4-azanyl-6-[1-(2-morpholin-4-ylethyl)pyrazol-4-yl]pyrimidine-5-carbonitrile | C14 H17 N7 O | 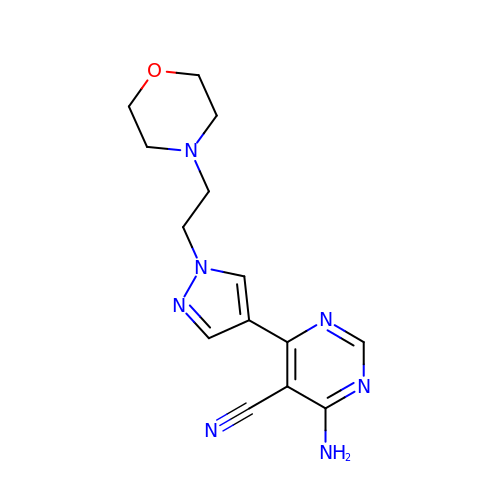DSZOJRUPLFLUKW-UHFFFAOYSA-N> GPVWRKHYITYRINNYTPDMNREDVDYAIRKAFQVWSNVTPLK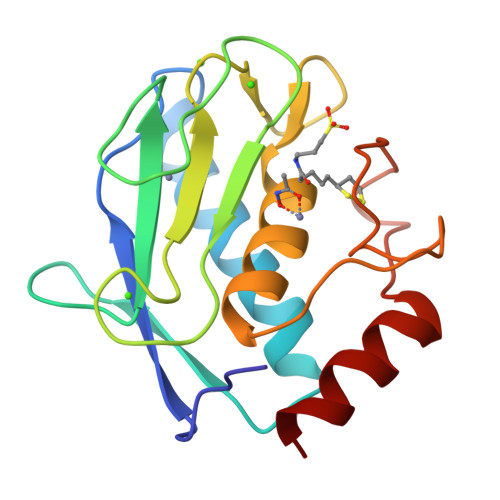FSKINTGMADILVVFARGAHGDDHAFDGKGGILAHAFGPGSGIGGDAHFDEDEFWTTHSGGTNLFLTAVHEIGHSLGLGHSSDPKAVMFPTYKYVDINTFRLSADDIRGIQSLYG>[3x]MK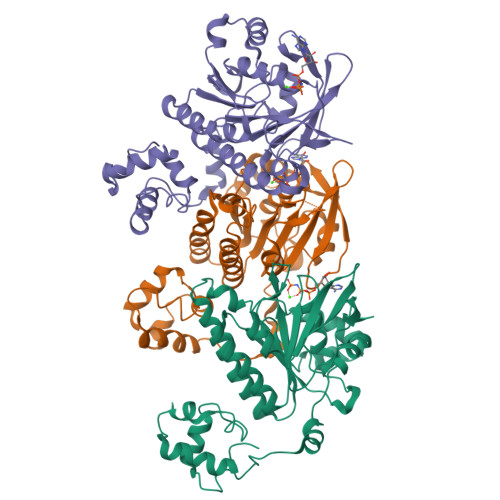EDQVVAEEPGFQDEEESLFQDIDLLQKHGINVADIKKLKSVGICTIKGIQMTTRRALCNVKGLSEAKVDKIKEAANKLIEPGFLTAFEYSEKRKMVFHITTGSQEFDKLLGGGIESMAITEAFGEFRTGKTQLSHTLCVTAQLPGAGGYPGGKIIFIDTENTFRPDRLRDIADRFNVDHDAVLDNVLYARAYTSEHQMELLDYVAAKFHEEAGIFKLLIIDSIMALFRVDFSGRGELAERQMKLAQMLSRLQKISEEYNVAVFVTNQMTADPGATMTFQADPKKPIGGHILAHASTTRISLRKGRGELRIAKIYDSPEMPENEATFAITAGGIGDAKE>[15x]DSQKWIVFLLFLIVLLQLAI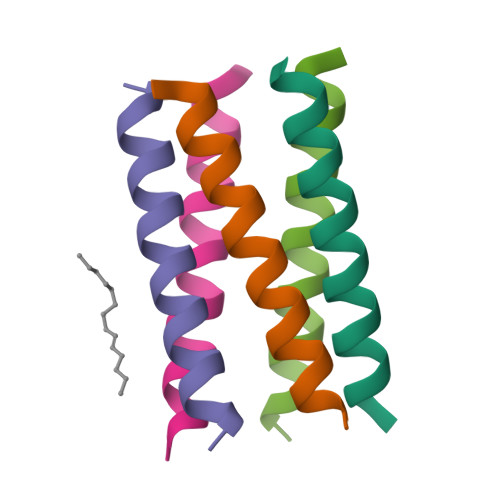VFLLRG> GPDFTKIIWPTVVERNFSNPQSEITTTLQELYGDTFETVSICPPQSYGGELLKGKIFFSSTPEFTREDLVEGKILASFKLDEVLSGLGMGAMLMTQIMSGHATIRVSAKVMLSKFCSFALKLVYDELMQLNSDTTDFGKISVLPGAIFSTQEEEFS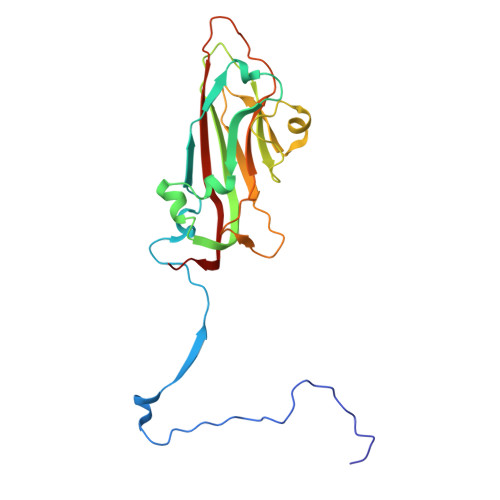FDFELFSPGVHLKFDNNKLLGKVHLAALSAPNLTENMPESFSCTFNFSIVDVKTTFYNIGQ> MHHHHHHSSGRENLYFQGSVEVHPVLEKLKAINNYNPKDFDWNLKNGRVFIIKSYCEDDIHRSIKYSIWCSTEHGNKRLDAAY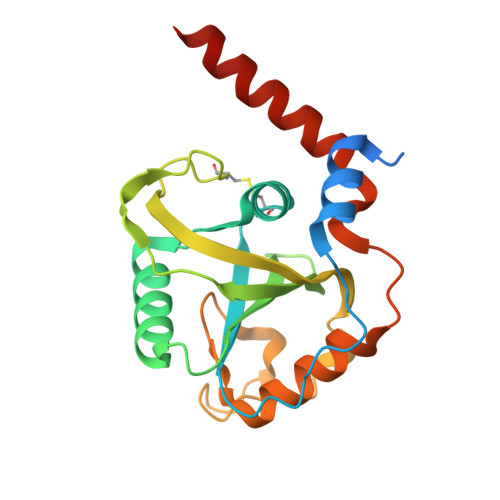RSLNGKGPLYLLFSVNGSGHFCGVAEMKSVVDYNAYAGVWCQDKWKGKFEVKWIFVKDVPNNQLRHIRLENNDNKPVTNSRDTQEVPLEKAKQVLKIIATFKHTTSIFDDFAHYEKRQEEEEAMRRERNRNKQ The SAM complex facilitates outer membrane β-barrel precursor protein folding and insertion into the outer membrane. The SAM complex consists of one copy each of Sam50, which spans the mitochondrial outer membrane, and Sam35 and Sam37, which sit on the cytosolic side of the membrane. Sam50 forms a 16-stranded β-barrel which is minimally closed between strands β1 and β16. The structures of Sam35 and Sam37 reveal that they each adopt a GST-like fold, which is also completely different from the BAM lipoproteins.

3D reconstructions for the SAM complex in GDN showed a mixture of monomers and three predominant dimer conformations. Among the dimer conformations, substantial differences were observed for the Sam50 β-barrel. However, in dimers 2 and 3, the β-barrel is open, allowing for association of strands β1 in an antiparallel arrangement, extending the β-sheet across two Sam50 β-barrels. A morph of Sam50 structures from dimers 1 and 3 shows how strands β1–β4 undergo an approximate 45° rotation, opening the β-barrel between strands β1 and β16 to create space for precursor protein to bind. In this morph between our observed conformations, strands β5–β16 remain mostly fixed, as does loop L6 and the conserved (V/I)RG(F/Y) motif. In Sam50, the barrel diameter by the POTRA domain stays constant while the upper ¾ region of strands β1–β4 can flip outward. All of the dimers appear to be non-physiological, with an up-down association of SAM complexes not anticipated from functional studies. Our structures illustrate how Sam50 can open sufficiently at the lateral gate to accommodate precursor binding at strand β1, positioning L6 at the lateral gate through its interaction(s) with strand β16.

>[2x]MASIPSAAPSWRKMQIPRPLQRLFDYFPLRIYEPNELPERSQQLTSGDLPTLYVFSTDSDARLGLPSFNPGCLKWQTLLRLANLDFRILPSTNHSSPTGSLPFLLPPRTSPTASPAPIPASGLLSFARKNPWRPGKAADLDLGHLDADLPPRAQAYLALITHSLRNAWLCALYLDPTHDALLRRLYVDPASSSRAVRAALLHQLRRAAAEQVATASSGGGKIVSLAPVDSADGIDEEAVYRSARDALDALASLLRESETAWFGTERPGSFDAALFSYTHLMVEYMSEEEDTESAKGRVSLGRMVKEAGNGELAEHRERMLGVAWPEWDGYRR;>[2x]MASSLGFGGSNAVDKVNATTTPGTVATPNSGPTKMLDEHILTPASISTLEVHGATNTRRSLLDQIFKPVLEDTAAAGTTLGQVLDRVGAATKKLARFDIFKEEGFGVFLSEAAPPQSAPPTDRTDLDISIRVKEKSRLVFSAGTDFGNAEGSAYTNAVVRNIFGGAETLTVNASTGTRTRSAYNATFSTPINGNPDLRLSVEALRSATQKPWASHEEHLTGANLRLAWLTEKGDTHALAYSSVWRQLTGLAPTASPTVRADAGDSLKSSLTHTFTRDRRDNPMLPQSGYLFRSVSELAGWGPLNGDVSFAKTEVEASGALPVAIPGLAGKSGVSVGGGLRLGVLYPLPLGYSLTGAAQPSRINDRFQLGGPNDVRGFKIGGLGPHDGVDAVGGDVFAAGSVNALLPLPRTGPDSPLRLQLYANAGRLVALNSKGTDKEGKEGLAMDSAAVFKGVKSAVGKLTNGIPSLAAGVGLVYAHPVARFELNFSLPLVLRRGEEGRKGLQVGVGISFL DsbA from E. coli K−12 (EcDsbA) was the first and is probably the best-characterised DSB enzyme to date. This 21 kDa periplasmic protein is a dithiol oxidase that catalyses disulphide bond formation between consecutive cysteines of unfolded polypeptides as they are translocated to the periplasm. EcDsbA consists of a canonical TRX domain, a hallmark of proteins involved in redox homeostasis, with an inserted helical domain. The TRX domain harbours the conserved active site CXXC (C30-P31-H32-C33 in EcDsbA) that is featured in many proteins of the TRX superfamily. The acidity of this groove originates from a cluster of negatively charged residues (E24, E37, E38, D44, E85, D86 and E94) that map along a buried channel in the interface between the TRX and helical domains of EcDsbA.

The other three mutants, E37A, E24A and E24A/E37A/K58A, were crystallised in space groups P21, P212121 and P2, respectively, with four molecules per asymmetric unit. The E24A mutant lacked the water-coordinating carboxyl group of the glutamic acid, which abolished the hydrogen bonding with water w3 and caused additional water molecules (w1’, w2’ and w3’) to occupy the space filled by the glutamic acid side chain in the native structure. In this structure, the K58 side chain shifts towards the E24-vacated space, and this change disrupts the proposed salt bridge between K58 and E37. Overall, in the E24A and E37A structures, although water molecules w1, w2 and w3 were still present and coordinated to the remaining charged residues in the channel, the number of interactions stabilising these water molecules was reduced, with the E37A mutant also resulting in the water network being less tightly connected to the bulk water (bw1/bw2). Water w4 was not observed in the crystal structures of any DsbA mutants, which is consistent with the relatively low conservation (42%) of this water molecule in the wildtype structures. E24A caused a 2.9-fold reduction in the initial rate, while K58A resulted in a 1.9-fold reduction in the initial rate. Intriguingly, E24A yielded a rate constant of 2.24 ± 0.14 × 106 M−1 s −1, almost identical to the wildtype. However, the double-mutant E24A/K58A yielded a rate constant of 1.47 ± 0.06 × 106 M−1 s −1, 35% slower than that of wildtype EcDsbA. These results indicated that E24A and K58A did influence DsbA oxidase activity, but its individual effect may be too small to be detected in this assay. Intriguingly, the effect of individual mutation E24A was undetectable in this in vivo assay. Cell-based assays showed that all DsbA mutants except E24A significantly affected ASST sulfotransferase activity in vivo, consistent with our in vitro data.

>AQYEDGKQYTTLEKPVAGAPQVLAFFSFFCPHCYQFEEVLHISDNVKKKLPEGVKMTKYHVNFMGGDLGKDLTQAWAVAMALGVEDKVTVPLFEGVQKTQTIRSASDIRDVFINAGIKGEEYDAAWNSFVVKSLVAQQEKAAADVQLRGVPAMFVNGKYQLNPQGMDTSNMDVFVQQYADTVKYLSEKK[4x]> GSAMDPGSGSGNSHNSLMKLL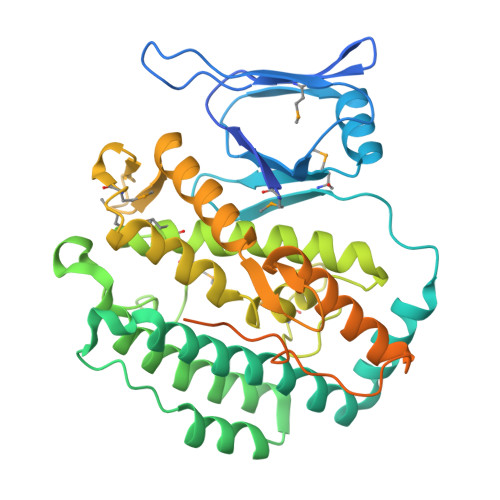LLNGHGINMHVDGAKLHIKDGRFSTTEEPQEYVFSPKRIDIDGIIIYGKSGNLTLEAIRWLIKHNVQVSILDWNGKLLTTMLPPESTNLRTKFAQYHAFEDKEARLEIAKKFIEAKFYKSKAVLDFLSQRYPEINFDILDGLTKLKDVKSTREILGVEGTLAGKYWIEFSKAVPKEYDFSNRIDQFRRAMGSGDMINTMLNYGYSLLEAECLKAINSVGLDTHVGFLHEMAPSKNSLAYDLQEPFRFIVDLAVISLIESGAMESKDFIRTENYNLRLKPTGARKIVNEFSNTLNKKVSYQGKESTWSYVIFLKVRELAHYLTSKKEKLDFTKPEYEIERIDSYDIRQKILSISYVDWKKLGFSKGTLHYMKQNAKSDKPFTLNAHVLERVNKWEALVSSQRDGRENLYFQ> NAAYYQVVPVTANVYDSDGEKLSYISQGSVVWLDKDRKSDDKRLAITISGLSGYMKTEDLQALDASKDFIPYYESDGHRFYHYVAQNASIPVASHLSDMEVGKKYYSADGLHFDGFKLENPFLFKDLTEATNYSAEELDKVFSLLNINN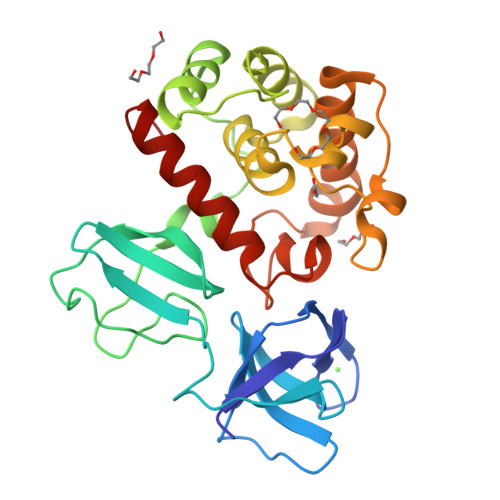SLLENKGATFKEAEEHYHINALYLLAHSALQSNWGRSKIAKDKNNFFGITAYDTTPYLSAKTFDDVDKGILGATKWIKENYIDRGRTFLGNKASGMNVEYASDPYWGEKIASVMMKINEKLGGKD> GMSIENLSSNKSFGGWHKQYSHVSNTLNCAMRFAIYLPPQASTGAKVPVLYWLSGLTCSDENFMQKAGAQRLAAELGIAIVAPDTSPRGEGVADDEGYDLGQGAGFYVNATQAPWNRHYQMYDYVVNELPELIESMFPVSDKRAIAGHSMGGHGALTIALRNPERYQSVSAFSPINNPVNCPWGQKAFTAYLGKDTDTWREYDASLLMRAAKQYVPALVDQGEADNFLAEQLKPEVLEAAASSNNY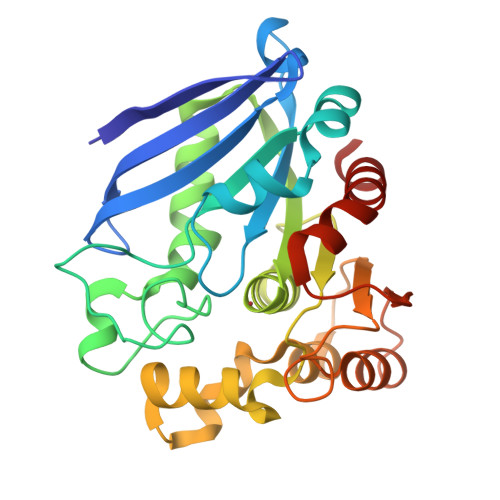PLELRSHEGYDHSYYFIASFIEDHLRFHSNYLNA> MRERPHTSGHHGAGEARATAPSTVSPYGPEARAELSSRLTTLRNTLAPATNDPRYLQACGGEKLNRFRDIQCRRQTAVRADLNANYIQVGNTRTIACQYPLQSQLESHFRMLAENRTPVLAVLASSSEIANQRFGMPDYFRQSGTYGSITVESKMTQQVGLGDGIMADMYTLTIREAGQKTISVPVVHVGNYPDQTAVSSEVTKALASLVDQTAETKRNMY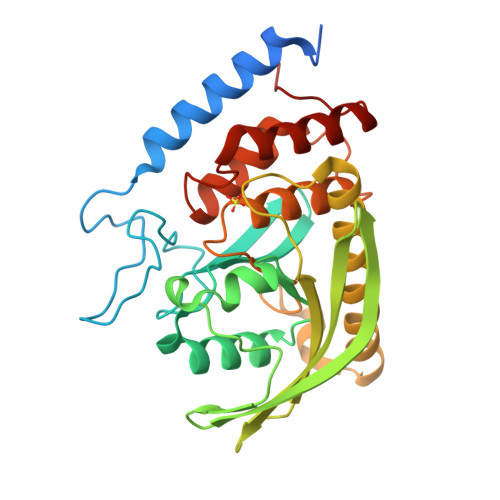ESKGSSAVADDSKLRPVIHCRAGVGRTAQLIGAMCMNDSRNSQLSVEDMVSQMRVQRNGIMVQKDEQLDVLIKLAEGQGRPLLNS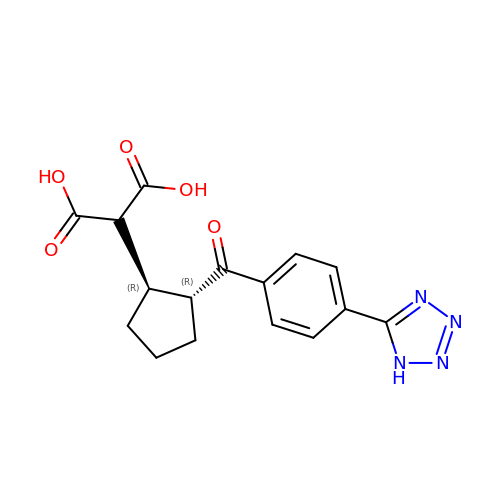{(1R,2R)-2-[4-(1H-tetrazol-5-yl)benzene-1-carbonyl]cyclopentyl}propanedioic acid | C16 H16 N4 O5 | DFKZAFCIROLDRJ-GHMZBOCLSA-N The causative agent for ASF is a DNA virus, African swine fever virus (ASFV). The polyprotein pp62 produces three mature structural proteins by the cleavage of viral protease pS273R, give rise to mature product p15, p35 and p8. Herein, we present the crystal structure of ASFV structural protein p35 (304 amino acid residues) and explore its potential role in core shell assembly. Membrane-associated proteins such as p35 may serve as a docking scaffold for the recruitment of host membrane and other components in the core shell during the virus assembly process and further stabilize the mature virion.

Due to the lack of a predicated homology model, the crystal structure of p35 is finally determined using single-wavelength anomalous diffraction (SAD) by a mercury (II) derivative and refined to 2.1  Å with a Rfactor and Rfree of 20.3% and 23.0%. While the high-resolution data were collected by the cube-like crystal grows in 0.1 mol/L BIS-TRIS pH 5.0, 25% w/v PEG 3350. In the final model, residues D1-Y11, D128-D138, G265-I273 and E299-N304 of Molecular A and B are not visible due to the lack of interpretable electron density data, suggesting their high structural flexibility. The ASFV p35 is a compact structure composed of eleven α-helices and four 310-helices. Homology search by the DALI server gives no structural homology with any identified proteins, indicating ASFV p35 as a completely novel fold structure. The structure of p35 can be described as two lobes of helix bundles, termed as a larger “head domain” and a relatively smaller “tail domain”, respectively. The head domain is a helix bundle with the central α4 surrounded by α1, α2, α3, α9 and α10, mainly stabilized by hydrophobic force, and further packed by α5, α8, and η1. The tail domain is a helix bundle composed by α6, α7, α11 and η4. In contrast, for ASFV p35, the two lobes are linked by three loops, rendering it as a much more compact structure. For ASFV p35, there are two charged patches in p35 protein surface: a continuous positive charged bulge composed of residues R16, R244, R278, and K168; and a negatively charged patch, which contains the residues D145, E147, E298, D227, and E232.

>RSPWDPPVPKHISPYTPRTRIAIEVEKAFDDCMRQNWCSVNNPYLAKSVSLLSFLSLNHPTEFIKVLPLIDFDPLVTFYLLLEPYKTHGDDFLIPETILFGPTGWNGTDLYQSAMLEFKKFFTQITRQTFMDIADSATKEVDVPICYSDPETVHSYTNHVRTEILHHNAVNKVTTPNLVVQAYNELEQTNTIRHYGPIFPESTINALRFWKKLWQDEQRFVIHGLHRTLMDQPTYETSEFAEIVRNLRFSRPGNNYINELNITSPAMYGDKHTTGDIAPNDRFAMLVAFINSTDFLYTAIPEEKVGGNLESRGPFEGKPIPNPLLGLDSTRTGHHHHHH[2x]> SGTGPGKSFCFATANVCLLPDSLARVNNLFNTQARAKEIGQRIRNGAARPQIKIYIDSPHPDEAFDHEVSAFFPANLDFLCLQEVFDKRAATKLKEQLHGYFEYILYDVGVYGCQGCCSFKCLNSGLLFASRYPIMDVAYHCYPNKCNDDALASKGALFLKVQVGSTPQDQRIVGYIACTHLHAPQEDSAIRCGQLDLLQDWLADFRKSTSSSSAANPEELVAFDVVCGDFNFDNCS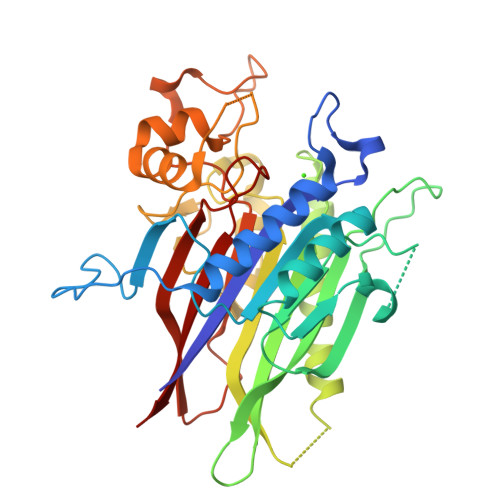SDDKLEQQHSLFTHYRDPCRLGPGEEKPWAIGTLLDTNGLYDEDVCTPDNLQKVLESEEGRREYLAFPTSKSSGQKGRKELLKGNGRRIDYMLHAEEGLCPDWKAEVEEFSFITQLSGLTDHLPVAMRLMVSSG> GPMTSQKLVRLPGLIDVHVHLREPGGTHKEDFASGTAAALAGGITMVCAMPNTRPPIIDAPALALAQKLAEAGARCDFALFLGASSENAGTLGTVAGSAAGLKLYLNETA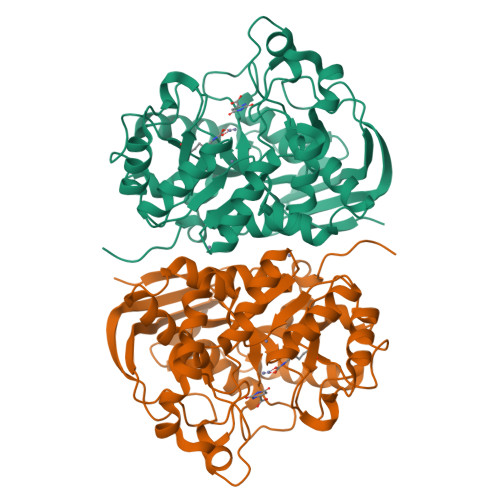SELRLDSVVQWMEHFETWPSHLPIVAHAEQQTVAAVLMVAQLTQRSVHICHVARKEEILLIKAAKARGLPVTCEVAPHHLFLSHDDLERLGPGKGEVRPELGSRQDVEALWENMAVIDCFASDHAPHTLEEKCGSRPPPGFPGLETMLPLLLTAVSEGRLSLDDLLQRLHHNPRRIFHLPPQEDTYVEVDLEHEWTIPSHMPFSKAHWTPFEGQKVKGTVRRVVLRGEVAYIDGQVLVPPGYGQDVRKWPQGAVPQLPPSAPATSEMTTTPERPRRGIPGLPD(3~{R})-1-[6-[(phenylmethyl)amino]pyrimidin-4-yl]-3-[[[6-[[(3~{S})-3-propan-2-yl-2-azoniaspiro[3.3]heptan-2-yl]methyl]naphthalen-1-yl]amino]methyl]piperidin-3-ol 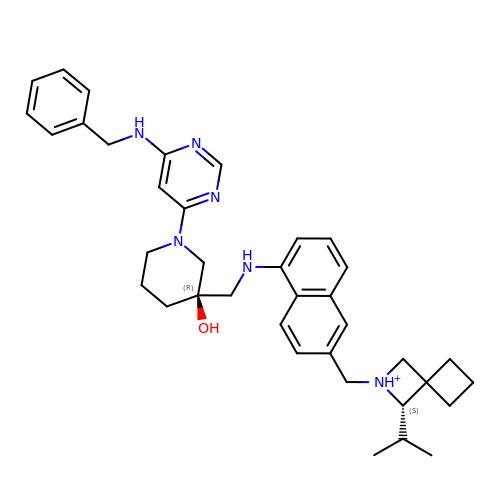| C37 H47 N6 O | DAMVLLAQUZPVCW-YBZKQSBQSA-O> M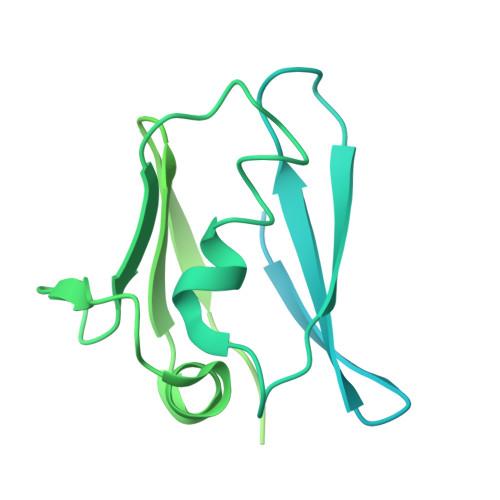AAAAGRSLLLLLSSRGGGGGGAGGCGALTAGCFPGLGVSRHRQQQHHRTVHQRIASWQNLGAVYCSTVVPSDDVTVVYQNGLPVISVRLPSRRERCQFTLKPISDSVGVFLRQLQEEDRGIDRVAIYSPDGVRVAASTGIDLLLLDDFKLVINDLTYHVRPPKRDLLSHENAATLNDVKTLVQQLYTTLCIEQHQLNKERELIERLEDLKEQLAPLEKVRIEISRKAEKRTTLVLWGGLAYMATQFGILARLTWWEYSWDIMEPVTYFITYGSAMAMYAYFVMTRQEYVYPEARDRQYLLFFHKGAKKSRFDLEKYNQLKDAIAQAEMDLKRLRDPLQVHLPLRQIGEKD> GAMDPEFMEMWHEGLE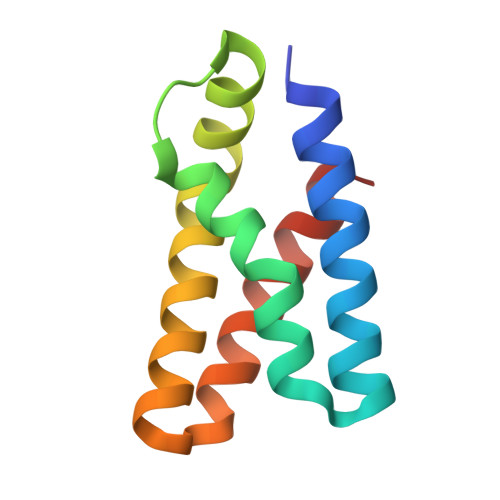EASRLYFGERNVKGMFEVLEPLHAMMERGPQTLKETSFNQAYGRDLMEAQEWCRKYMKSGNVKDLTQAWDLYYHVFRRISKQ> MSAEKLFTPLKVGAVTAPNRVFMAPLSRLRSIEPGDIPTPLMGEYYRQRASAGLIISEATQISAQAKGYAGAPGLHSPEQIAAWKKITAGVHAEDGRIAVQLWHTGRISHSSIQPGGQAPVSASALNANTRTSLRDENGNAIRVDTTTPRALELDEIPGIVNDFRQAVANAREAGFDLVELHSAHGYLLHQFLSPSSNQRTDQYGGSVENRARLVLEVVDAVCNEWSADRIGIRVSPIGTFQNVDNGPNEEADALYLIEELAKRGIAYLHMSETDLAGGKPYSEAFRQKVRERFHGVII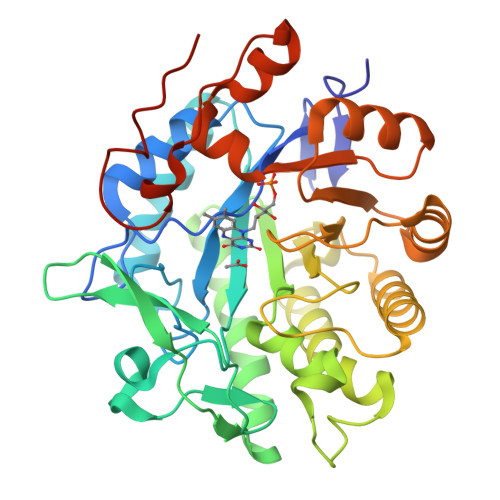GAGAYTAEKAEDLIGKGLIDAVAFGRDYIANPDLVARLQKKAELNPQRPESFYGGGAEGYTDYPSLHHHHHHHH> HQHGVVYITENKNKTVVIPCLGSISNLNVSLCARYPEKRFVPDGNRISWDSKKGFTIPSYMISYAGMVFCEAKINDESYQSIMYIVVVVGYRIYDVVLSPSHGIELSVGEKLVLNCTARTELNVGIDFNWEYPSSKHQHKKLVNRDLKTQSGSEMKKFLSTLTIDGVTRSDQGLYTCAASSGLMTKKNSTFVRVHEKPF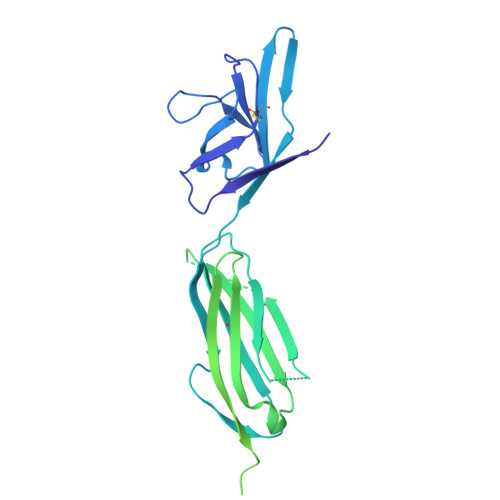VAFGSGMESLVEATVGERVRIPAKYLGYPPPEIKWYKNGIPLESNHTIKAGHVLTIMEVSERDTGNYTVILTNPISKEKQSHVVSLVVYVPPQIGEKSLISPVDSYQYGTTQTLTCTVYAIPPPHHIHWYWQLEEECANEPSQAVSVTNPYPCEEWRSVEDFQGGNKIEVNKNQFALIEGKNKTVSTLVIQAANVSALYKCEAVNKVGRGERVISFHRTHHHHHH>GAMSIFDKRVNYKPFEYPEVLQFTEAINKAYWVHTEVDFTADTQDFHAHLSLAEKTAVKNSLLAIAQIEVAVKSFWGNIYEHFPKPEFNGLGSTFAECEFRHSEAYSRLLEVLGYNDEFEKLLDVPVIRRRVDYLSNVLKDTKSQDNRKYMVSLILFSILIENV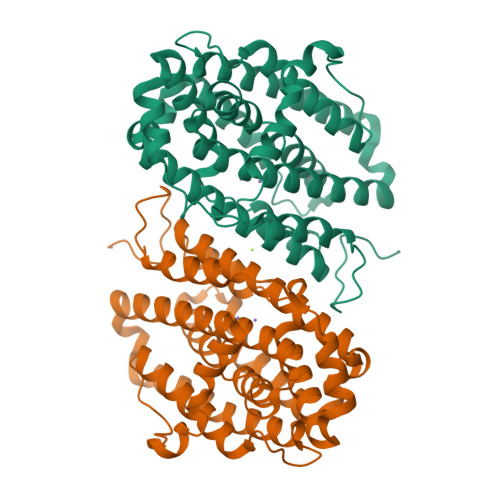SLFSQFAILLSFTRFKGYMKNVSNIIAWTSIDEQIHANGGIYIINKIREEFPDYFDEETLALVRETVKDSIAVESDILDWIFEEGEIESIKKGDLVNFMKFRIDESLKQINIPVIFDVKVEDYKALAWFEEEVFANSLDDFFAK[2x]>SNAERKEGEVAGLDMNISQFLKSLGLEHLRDIFETEQITLRVLADMGHEELKEIGINAYGHRHKLIKGVERLLGGQQGT[6x]

The poly(ADP-ribose) polymerases (PARPs) Tankyrase (TNKS and ARTD5) and Tankyrase 2 (TNKS2 and ARTD6) regulate Wnt-β-catenin signaling (Huang et al., 2009). The two Tankyrases are highly similar (Hsiao and Smith, 2008, Smith et al., 1998), sharing a set of five ankyrin repeat clusters (ARCs) for substrate binding (Guettler et al., 2011, Seimiya et al., 2004), a sterile alpha motif (SAM) domain (De Rycker and Price, 2004, De Rycker et al., 2003), and a catalytic PARP domain (Rippmann et al., 2002). Tankyrase polymerization is mediated by the SAM domain, a small helical fold highly prevalent in eukaryotes (Knight et al., 2011, Qiao and Bowie, 2005). We report crystal structures of the polymerizing TNKS and TNKS2 sterile alpha motif (SAM) domains, revealing versatile head-to-tail interactions.

We also crystallized the TNKS SAM domain, which again required a polymer-breaking mutation. TNKS SAM D1055RT1, equivalent to D902RT2, produced two crystal forms in space group P21, diffracting to 2.5 Å (crystal form 1) and 2.9 Å (crystal form 2), both with six molecules in distinct asymmetric units. The TNKS SAM domain was highly similar to that of TNKS2 (left). For both TNKS crystal forms, non-crystallographic and crystallographic symmetry gave rise to left-handed helical filaments established by EH-ML contacts. The repeating unit consisted of six SAM domains with pitches of 83 and 79 Å, almost twice as long as for TNKS2. Unlike for TNKS2, where protomer contacts relied on crystallographic symmetry only and were therefore uniform, the TNKS SAM EH-ML contacts varied substantially. This was apparent from the merely approximate 6-fold axial symmetry and the variable tilt and twist between adjacent SAM domains. We conjecture that the variable relative orientations of SAM domains reflect filament flexibility. However, the equivalent residues (D1059T1, K1066T1, and K1081T1, respectively) mediated binding between a subset of protomers in the TNKS SAM crystal structures. Thus, contacts not seen in all SAM-SAM pairs are still generally relevant, probably occurring in some, but not all, configurations of the flexible filament.> MASSINPW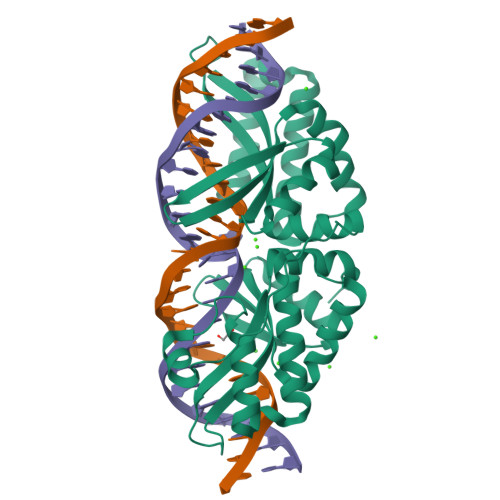ILTGFADAEGSFLLRIRKYSQTRVGYLTELGFQITLHNKDKSILENIQSTWGVGVIANSGDNAVSLKVTRFEDLKVIIDHFEKYPLITQKYADYMLFKQAFNVMENKEHLTIEGIKELVRIKAKLNWGLTDELKKAFPEIISKERSLINKNIPNFKWLAGFTSGDGCFFVNLSKKKTKLGVQVKLVFSISQHIRDKNLMNSLITYLGCGYIKKKNKSEFSWLEFVVTKFSDIRDKIIPFFQEYTLIGTKLKDFEDWCKVAKLIEEKKHLTEEGLDEIKKIKLNMNKGR> ELTPDQQTLLHFIMDSYNKQRMPQEITNKILK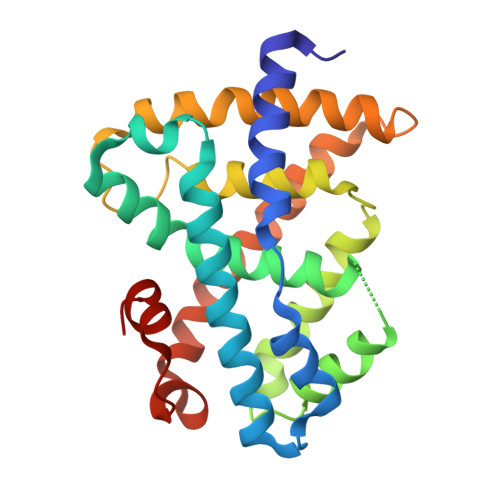EEFSAEENFLILTEMATNHVQVLVEFTKKLPGFQTLDHEDQIALLKGSAVEAMFLRSAEIFNKKLPSGHSDLLEERIRNSGISDEYITPMFSFYKSIGELKMTQEEYALLTAIVILSPDRQYIKDREAVEKLQEPLLDVLQKLCKIHQPENPQHFACLLGRLTELRTFNHHHAEMLMSWRVNDHKFTPLLCEIWDVQ> GSSQNEASEDTGFNPKAFPLASPDLNNKIINLVQQACNYKQLRKGANEATKALNRGIAEIVLLAADAEPLEILLHLPLVCEDKNTPYVFVRSKVALGRACGVSRPVIAAAITSKDGSSLSSQITE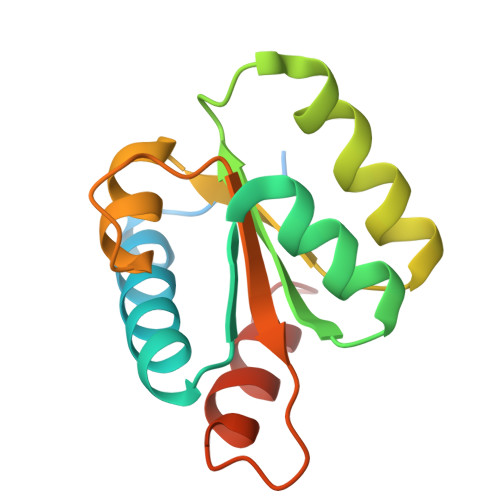LKDQIEQILV>MGSSHHHHHHSSGLVPAGSHSKVFIRSAINRVHQNSAANGGELPRIVFPEGTSTKVLKALATLVEEKICQPILLGYPERVKEKIKALDIPLLNDVSIVHPSSHPKYFSFVEKLYSLRQRKGINLGEAERLMADPNYFAAMMVNQGEADGMVSGSSINYADAVRPILQTIGVYKEGIPAGLNFVLLEDKFLVLADTTVNLNPTAEQCAQIALQAAKIVEYFGIEPRVAMLSYSNFSGAEGTPRKMKKAAEIARSLRPDLMIEGDMQADTAVNPEIMERLFPFSGLKGGANVLVFPNLESSNIAYKLIQQIGKAEVI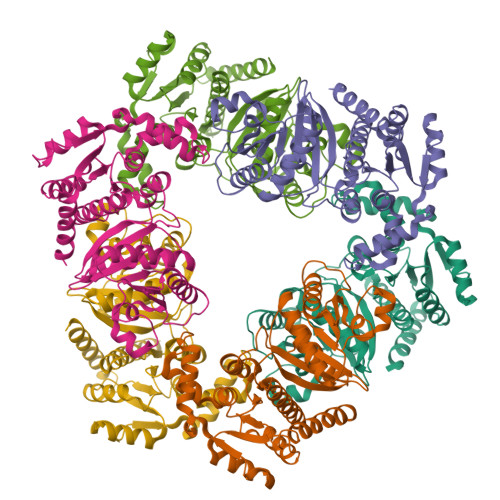GPFLTGVRRSANVLQRTTTVDGIVNSVVFTALEAQYIKEVLKSRGKK[12x]> GSFMKTIGIFYATLTKTTVGIVDEIEFFLKKDDFKTFNVKNGVKEIENFENLILVTPTYQVGEAHAAWMNNLKKLEEIDFTGKVVGLVGLGNQFAFGESFCGGIRYLYDIVVKKGGKVVGFTSTDGYHYEETSIIE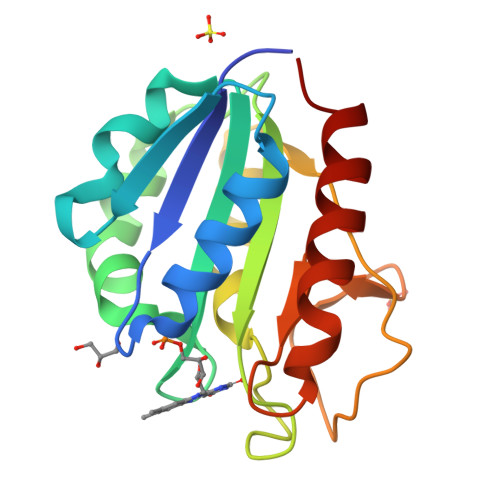NGKFIGLALDEENQPNLTPKRIGDWITEIKKEFK>MGSSHHHHHHSSGRENLYFQGPSLLLSKRIIFLSSPIYPHISEQIISQLLYLEYESKRKPIHLYINSTGDIDNNKIINLNGITDVISIVDVINYISSDVYTYCLGKAYGIACILASSGKKGYRFSLKNSSFCLNQSYSIIPFNQATNIEIQNKEIMNTKKKVIEIISKNTEKDTNVIS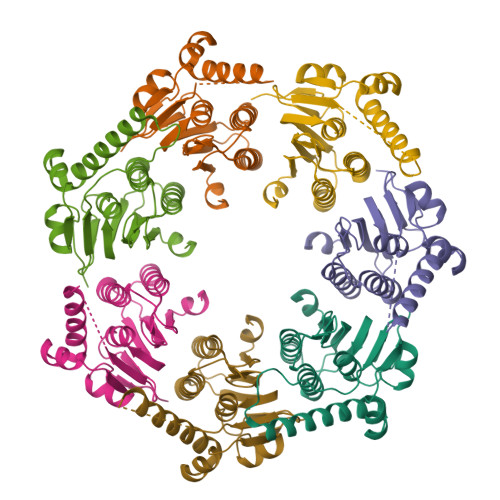NVLERDKYFNADEAVDFKLIDHILEKE[7x]> SRHSEKIAIRDFQVGDLVLIILDERHDNYVLFTVSPTLYFLHSESLPALDLKPG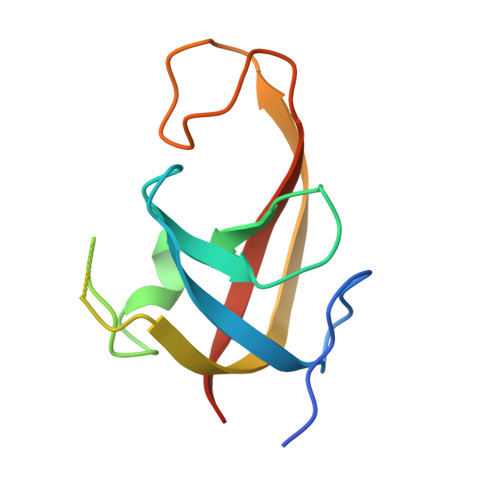EGASGASRRPWVLGKVMEKEYCQAKKAQNRFKVPLGTKFYRVKAVSWNKKV>[2x]MSLKTTTSSTP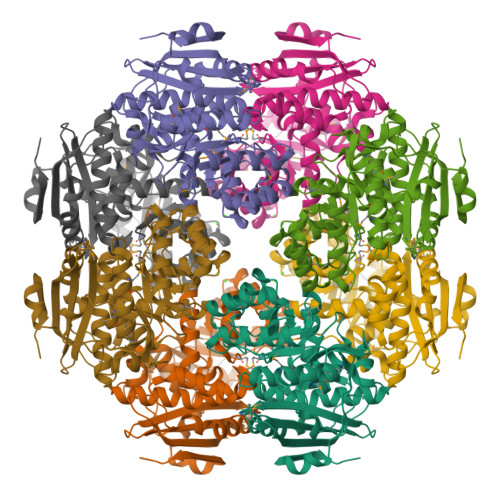SDRITWVRISSCYLPLATPISDAKVLTGRQKPMTEIAILFAEIETAGGHQGLGFSYSKRAGGPGQFAHAREIAPALIGEDPSDIAKLWDKLCWAGASAGRSGLSTQAIGAFDVALWDLKAKRAGLSLAKLLGSYRDSVRCYNTSGGFLHTPIDQLMVNASASIERGIGGIKLKVGQPDGALDIARVTAVRKHLGDAVPLMVDANQQWDRPTAQRMCRIFEPFNLVWIEEPLDAYDHEGHAALALQFDTPIATGEMLTSAAEHGDLIRHRAADYLMPDAPRVGGITPFLKIASLAEHAGLMLAPHFAMELHVHLAAAYPREPWVEHFEWLEPLFNERIEIRDGRMLVPTRPGLGLTLSGQVKAWTREEAQVGTRPEGHHHHHH> MPYAGEGSNPLGLKDFLDDLRLDHYQDLLRELDELYQKLKQERQVPLHGDGEAYPLLTLTVDGGEGRAFEELPLLSFGLVRVAAVGVKGFRLPSIA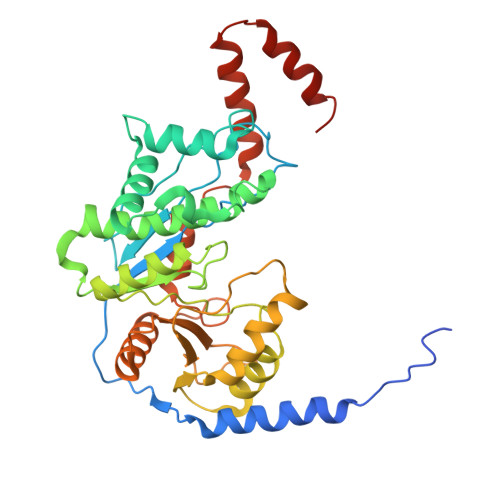HLLPGYEVLRDPKGYLEGLLERSEESPAADALKTFFRATGISLEDLGEYYTKDLRAFMGIFRDVLEWAYLVWGVEKVLQESYKDYLFIKDGRLAQLGVRESFRSKLQNYFARKHLLLAGVTKRSRLLAEGLTSLVMARLFAEARGTFVLQVPQELMEKAYRYERQWNADLEGAFVMGRRYVARLLEDTFRPQEGVAIFDLPPYLGEEDAVKVARSLRAHRSVLYGGSVGTVVEAHGRASVARSIPRRMEEEILARFRKAFGEDLAKKLTEWLRLADRED DNA ligases are enzymes which join breaks in the phosphodiester backbone of double-stranded DNA using an adenylate-donating cofactor: either ATP or NAD+. The ATP-dependent class of DNA ligases are widespread in biology and are found in all archaea and eukaryotes as well as a large number of bacteria and viruses. Here, we present the crystal structure of the ATP-dependent DNA ligase from Rhizobium phage vB_RleM_P10VF (P10VF-Lig), which has substantial structural similarity to T4 DNA ligase as well as to the ATP-dependent DNA ligase from the cyanobacterium Prochloro­coccus marinus (Pmar-LigP), despite having low overall sequence identity to either protein.

Here, we report the crystal structure of the ATP-dependent DNA ligase from the Rhizobium phage vB_RleM_P10VF bound to a nicked DNA duplex determined to 2.2 Å resolution. The P10VF-Lig DNA ligase was crystallized in the closed conformation bound to nicked DNA. Analysis of the overall structure revealed that the DNA duplex was encircled by the three globular domains: the highly conserved NTase domain, C-terminal OB domain and N-terminal DB domain. The NTase domain of T4 DNA ligase also contains additional helical elements relative to P10VF-Lig which insert into the minor groove on the 3′-end of the DNA nick. In P10VF-Lig the equivalent 17 residues between Ala212 and Asn229 have no visible density. To this end, P10VF-Lig and a second novel phage-derived T4-DNA ligase homolog from Acinetobacter phage Ac42 (Ac42-Lig) were assayed on a range of ligatable DNA substrates and compared with T4 DNA ligase and the bacterial ATP-dependent DNA ligase Pmar-LigP. Despite the relatively high structural similarity between P10VF-Lig and T4 DNA ligase, P10VF-Lig exhibited considerably lower specific activity on most substrates tested, with no detectable ligation on cohesive overhangs.

> GLDIFSDNVSEINRISDIINSDLQAIADSKGTNAKKVELAKISEYTFKCFVFHLDPFQNFGISKLSKDAGGGEGIDWSTVFKLLYEGKGRDLKKRDKSLTTLQAKIINGIFDGFMDWKPGVKGGSFLDVFPDSYRTFEVQKCANWDPDLFEANSFAQIKFDGIRCVAMVDHNGNLTYVSRNGKPVVNIDPRIEENMKLHPGWCFDAEADSPAKFQKTSGISRASKSGSNIKLTLRVFDAIPYDAFLARKYDVQYIERYNDLKSMWSNNPFLFDLIADHTLVETWEDAQKFYEDSRANGNEGAIVKKRFGTYNFGRDDSWMKVKPLETIEARIIGYEEGKPKTKHVGRVGALIVQDYTGAISRVGSGMSDKERQYIYDNWDEFENALCEVKFMERTESGVFRHSRLSKIRLDKDDMNPTGA>[4x]AMASSESAFLAQHGLAGKTVEQIVDTIDQTPQSRPLPYSASITSTELKLSDGEQIYTLPLGDKFYLSFAPYEWR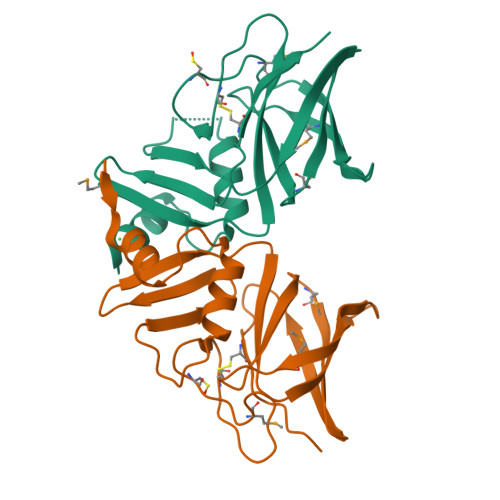THPCFNHSLSGCQGEMPNKPFTVKVTDSKGAVIVQKEMQSYRNGFIGVWLPRNMEGTLEVSYNGKTASHAIATSDDSQTCLTELPLR> AAAAAAAAAAAAAAAAAAAAAAAAAAAAAAAAAAAAAAAAAA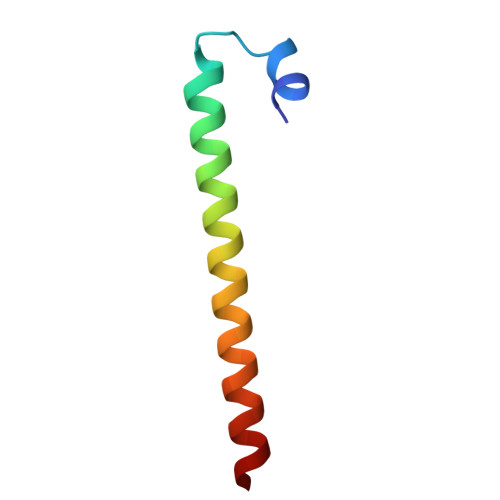AAAAAAA>[4x]GPGSMKQYLDLVRTILDTGTWQSNRTGIRTIGIPGAMLRFDLQQGFPAVTTKKLAFKSAIGELVGFLRATRSAAEFRALGCKVWDANANENAQWLANPYRRGADDLGDVYGVQWRRWPGYKVLDAHADAQIADATSRGFRIVAR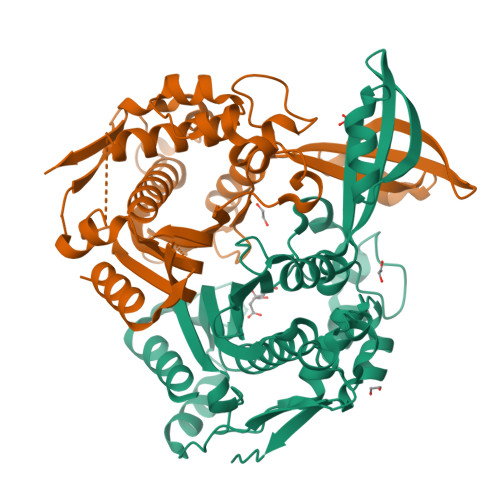FEEGGADKVLLHKAIDQLRDCLDTIVRDPSSRRILFHGWNPAVLDEIALPACHLLYQFLPNVERREISLCLYIRSNDVGLGTPFNLAEGAALLTLVGRLTGYSPRWFTYFIGDAHIYENQLDMLKQQLEREPFESPRLELAERVPDYAKTGKYEPQWLERVEPSDFTLVGYRHHEPLSAPMAV MnmE and MnmG form a conserved protein complex responsible for the addition of a 5-carboxymethylaminomethyl (cmnm) group onto the wobble uridine of several transfer RNAs (tRNAs). Within this complex, both proteins collaborate intensively to catalyze a tRNA modification reaction that involves glycine as a substrate in addition to three different cofactors, with FAD and NADH binding to MnmG and methylenetetrahydrofolate (5,10-CH2-THF) to MnmE. MnmE is a homodimeric protein of 50–55 kDa subunits, with each protomer composed of three discernable domains: an N-terminal domain required for constitutive dimerization and binding of 5,10-CH2-THF, a helical domain and a Ras-like GTPase domain (G domain) that is inserted in the helical domain. Within the MnmEG complex, MnmG is responsible for binding the cofactors FAD and NADH, and it is also the main driver for binding of the tRNA substrate.

However, upon binding of K+ and GTP, MnmE and MnmG adopt an elongated α4β2 complex, where one MnmG dimer is flanked on each side by an MnmE dimer. In the α4β2 complex, the vacant MnmG subunit is occupied by a second MnmE dimer, resulting in an even more elongated arrangement. This configuration results in two vacant MnmE subunits on each side of the α4β2 oligomer. Homogeneous refinement, followed by NU-refinement resulted in a 3.3 Å map reconstruction for the α2β2 complex using C1 symmetry, and a 4.0 Å map for the α4β2 complex using C2 symmetry. To build the α4β2 complex, first the MnmE asymmetric dimer was taken from the α2β2 model and fitted in an identical fashion in the region of the α4β2 map corresponding to the MnmE A and B subunits (with MnmE subunit B interacting with MnmG subunit C). In the same way, MnmE was placed in the region of the map corresponding to the MnmE E and F subunits (with MnmE subunit E interacting with MnmG subunit D). Correspondingly, in the α4β2 complex both α-helical domains of the MnmG dimer are structured upon interaction with MnmE, and the symmetry in MnmG is restored. In the α4β2 complex similar conformational changes, albeit at lower resolution, can be observed between the subunits (A versus B or E versus F) of both MnmE molecules bound at either side of MnmG. Also for the resulting α4β2 complex we find a good fit with the SAXS data of the corresponding complex in solution, with a χ2 value of 2.6.

>[4x]MSDNDTIVAQATPPGRGGVGILRISGFKAREVAETVLGKLPKPRYADYLPFKDADGSVLDQGIALWFPGPNSFTGEDVLELQGHGGPVILDLLLKRILTIPGLRIARPGEFSERAFLNDKLDLAQAEAIADLIDASSEQAARSALNSLQGAFSARVNHLVEALTHLRIYVEAAIDFPDEEIDFLSDGKIEAQLNDVIADLDAVRAEARQGSLLREGMKVVIAGRPNAGKSSLLNALAGREAAIVTDIAGTTRDVLREHIHIDGMPLHIIDTAGLREASDEVERIGIERAWQEIEQADRVLFMVDGTTTDAVDPAEIWPEFIARLPAKLPITVVRNKADITGETLGMSEVNGHALIRLSARTGEGVDVLRNHLKQSMGFDTNMEGGFLARRRHLQALEQAAEHLQQGKAQLLGAWAGELLAEELRLAQQNLSEITGEFTSDDLLGRIFSSFCIGK;>[2x]MGSSHHHHHHSSGENLYFQGMFYPDPFDVIIIGGGHAGTEAAMAAARMGQQTLLLTHNIDTLGQMSCNPAIGGIGKGHLVKEVDALGGLMAKAIDQAGIQFRILNASKGPAVRATRAQADRVLYRQAVRTALENQPNLMIFQQAVEDLIVENDRVVGAVTQMGLKFRAKAVVLTVGTFLDGKIHIGLDNYSGGRAGDPPSIPLSRRLRELPLRVGRLKTGTPPRIDARTIDFSVLAQQHGDNPMPVFSFMGNASQHPQQVPCYITHTNEKTHDVIRSNLDRSPMYAGVIEGVGPRYCPSIEDKVMRFADRNQHQIFLEPEGLTSNEIYPNGISTSLPFDVQMQIVRSMQGMENAKIVRPGYAIEYDFFDPRDLKPTLESKFIQGLFFAGQINGTTGYEEAAAQGLLAGLNAARLSADKEGWAPARSQAYLGVLVDDLCTLGTKEPYRMFTSRAEYRLMLREDNADLRLTEIGRELGLVDDERWARFNEKLENIERERQRLKSTWVTPSAEAAAEVNAHLTAPLSREASGEDLLRRPEMTYEKLTTLTPFAPALTDEQAAEQVEIQVKYEGYIARQQDEIEKQLRNENTLLPATLDYRQVSGLSNEVIAKLNDHKPASIGQASRISGVTPAAISILLVWLKKQGMLRRSA>[8x]MKIA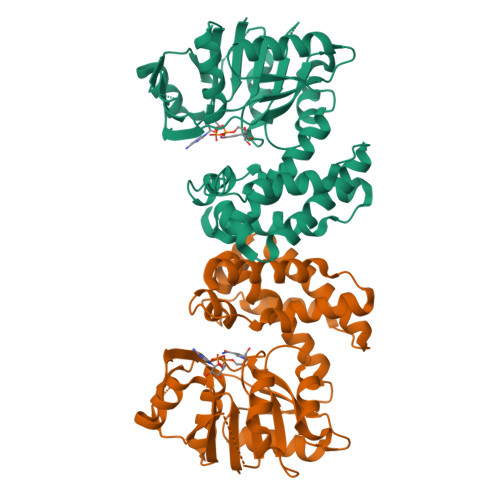IAGAGAMGSRFGLMLHQSGNEVLLIDGWAEHVQQIKEHGLQANFNGKEVEAKLPIVLQSEVEKEDQVDLIILFTKAMQLEKMLQDIQSLIKKDTEVLCLLNGIGHEDIIEKFVPMENIYIGNTMWTAGLEGPGQVKLFGSGSVELQNLGDGKEAAAKKLADKLSESGLNAHFSDNIHYSIYRKACVNGTMNGLCTILDVNMAELGKTSTAHKMVATIVNEFAKVAAVEKIELDVPEVIAHCESCFDPETIGLHYPSMYQDLIKNHRLTEIDYINGAISRKGKKYGVATPYCDFLTELVHAKEDSLNVK> RIRALPAAPGVAIAEGWQDATLPLMEQVYQASTLDPALERERLTGALEE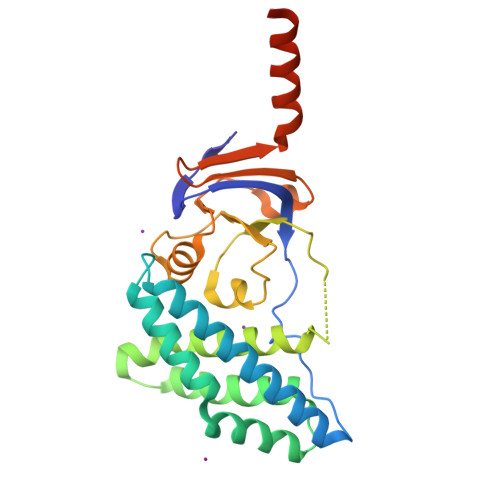AANEFRRYSKRFAAGAQKETAAIFDLYSHLLSDTRLRRELFAEVDKGSVAEWAVKTVIEKFAEQFAALSDNYLKERAGDLRALGQRLLFHLDDANQGPNAWPERFILVADELSATTLAELPQDRLVGVVVRDGAANSQAAIMVRALGIPTVMGADIQPSVLHRRTLIVDGYRGELLVDPEPVLLQEYQRLISEEIELSRLAEDDVN> MSSLINHAMSGLNAAQAALNTVSNNINNYNVAGYTRQTTILAQANSTLGAGGWIGNGVYVSGVQREYDAFITNQLRGAQNQSSGLTTRYEQMSKIDNLLADKSSSLSGSLQSFFTSLQTLVSNAEDPAARQALIGKAEGLVNQFKTTDQYLRDQDKQVNIAIGSSVAQINNYAKQIANLNDQISRMTGVGAGASPNDLLDQRDQLVSELNKIVGVEVSVQDGGTYNLTMANGYTLVQGSTARQLAAVPSSADPTRTTVAYVDEAAGNIEIPEKLLNTGSLGGLLTFRSQDLDQTRNTLGQLALAFADAFNAQHTKGYDADGNKGKDFFSIGSPVVYSNSNNADKTVSLTAKVVDSTKVQATDYKIVFDGTDWQVTRTADNTTFTATK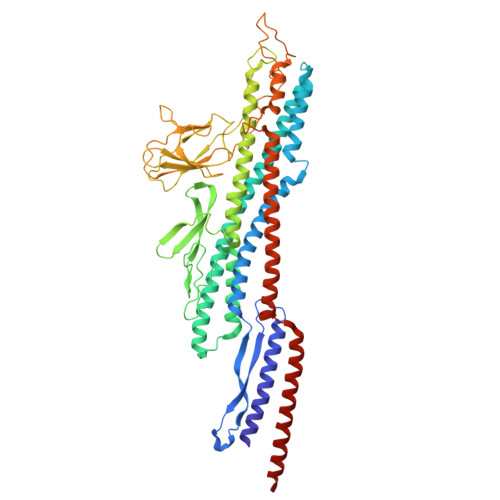DADGKLEIDGLKVTVGTGAQKNDSFLLKPVSNAIVDMNVKVTNEAEIAMASESKLDPDVDTGDSDNRNGQALLDLQNSNVVGGNKTFNDAYATLVSDVGNKTSTLKTSSTTQANVVKQLYKQQQSVSGVNLDEEYGNLQRYQQYYLANAQVLQTANALFDALLNIR> ADYDLKFGMNAGTSSNEYKAAEMFAKEVKEKSQGKIEISLYPSSQLGDDRAMLKQLKDGSLDFTFAESARFQLFYPEAAVFALPYVISNYNVAQKALFDTEFGKDLIKKMDKDLGVTLLSQAYNGTRQTTSNRAINSIADMKGLKLRVPDAATNLAYAKYVGASPTPMAFSEVYLALQTNAVDGQENPLAAVQAQKFYEVQKFLAMTNHILNDQLYLVSNETYKELPEDLQKVVKDAAENAAKYHTKLFVDGEKDLVTFFEKQGVKITHPDLVPFKESMKPYYAEFVKQTGQKGESAL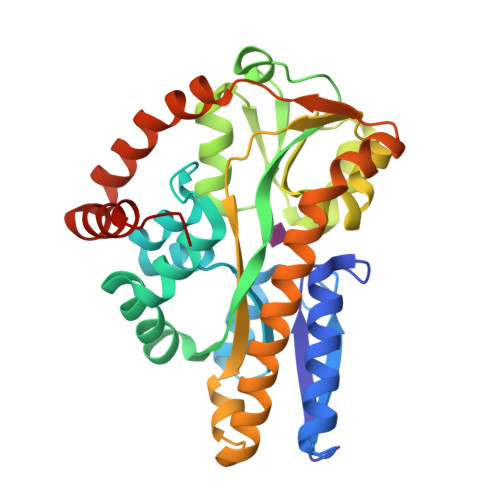KQIEAINPHHHHHH> 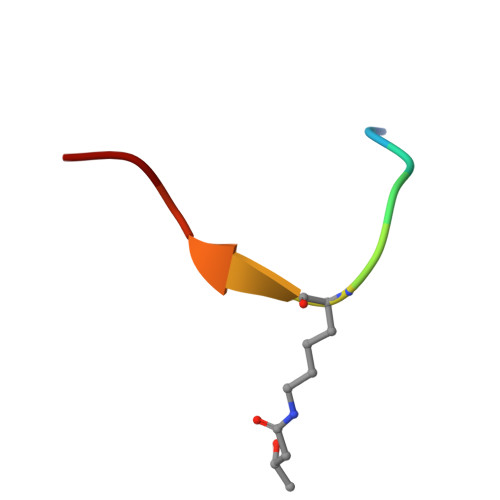GKGGAXRHRKV> MDLATLLGLIGGFAFVIMAMVLGGSIGMFVDVTSILIVVGGSIFVVLMKFTMGQFFGATKIAGKAFMFKADEPEDLIAKIVEMADAARKGGFLALEEMEINNTFMQKGIDLLVDGHDADVVRAALKKDIALTDERHTQGTGVFRAFGDVAPAMGMIGTLVGLVAMLSNMDDPKAIGPAMAVALLTTLYGAILSNMVFFPIADKLSLRRDQ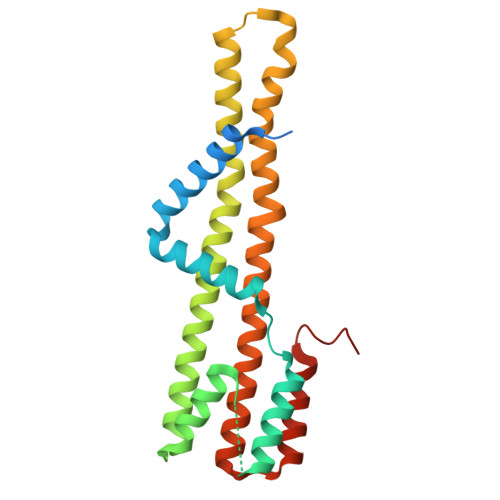ETLNRRLIMDGVLAIQDGQNPRVIDSYLKNYLNEGKRALEIDE Target-based azole resistance in Candida albicans involves overexpression of the ERG11 gene encoding lanosterol 14α-demethylase (LDM), and/or the presence of single or multiple mutations in this enzyme. The azole antifungals inhibit sterol 14α-demethylase (CYP51, SDM), thereby preventing biosynthesis of the essential and fungal specific sterol ergosterol, and resulting in the collateral synthesis of toxic sterols. We have used, as surrogates, structurally aligned mutations in recombinant hexahistidine-tagged full-length Saccharomyces cerevisiae LDM6×His (ScLDM6×His) to elucidate how differential susceptibility to azole drugs is conferred by LDM of the C. albicans Darlington strain. Phenotypes and high-resolution X-ray crystal structures were determined for the surrogate enzymes in complex with representative short-tailed (voriconazole) and long-tailed (itraconazole) triazoles.

Boat-shaped crystals of Ni-NTA affinity and size exclusion chromatography (SEC) purified ScLDM6×His Y140H in complex with VCZ formed after 15 days in 46% PEG, 0.5 M glycine pH 9.6. However, no active site water molecule was detected within 5 Å of VCZ in this 1.9 Å resolution structure, and the VCZ was displaced slightly towards H140 and helix I by <0.5 Å. Thus, there are no water-mediated hydrogen bond networks involving the tertiary alcohol of VCZ and Y140H and the heme ring D propionate, or between the 5-fluoropyrimidine ring and the main chain nitrogen of S382 and the main chain carbonyl of M509, as was found with the wild-type enzyme. The significantly different disposition of M509 between the wild-type and Y140H structures may be due to the absence of this water-mediated hydrogen bond network. There is also a significant impact on the disposition of Y126, which neighbors Y140/H, as the 5-fluoropyrimidine ring of VCZ was flipped 180 degrees between the wild-type and Y140H mutant structure. While the Y126 sidechain hydroxyl retained a hydrogen bond with the main chain amide of F384 in ScLDM6×His Y140H, a hydrogen bond with the heme ring D propionate was not formed. Due to the movement of VCZ towards helix I and the mutated histidine, the Y140H mutation ablates a key water-mediated hydrogen bond network involving the VCZ 5-fluoropyrimidine, the main chain amide of S382, and the main chain carbonyls of M509. While the ionic interactions of the heme with K151 and R385 were retained in ScLDM6×His Y140H, the loss of hydrogen bonds between Y140 and the heme ring C propionate, and between Y126 and the heme ring D propionate may be expected to affect the electronic status of the heme. This interpretation is consistent with the slight (1 nm) red shift from 417 nm to 418 nm in the main Soret peak of ScLDM6×His Y140H.

> MSATKSIVGEALEYVNIGLSHFLALPLAQRISLIIIIPFIYNIVWQLLYSLRKDRPPLVFYWIPWVGSAVVYGMKPYEFFEECQKKYGDIFSFVLLGRVMTVYLGPKGHEFVFNAKLADVSAEAAYAHLTTPVFGKGVIHDCPNSRLMEQKKFVKGALTKEAFKSYVPLIAEEVYKYFRDSKNFRLNERTTGTIDVMVTQPEMTIFTASRSLLGKEMRAKLDTDFAYLYSDLDKGFTPINFVFPNLPLEHYRKRDHAQKAISGTYMSLIKERRKNNDIQDRDLIDSLMKNSTYKDGVKMTDQEIANLLIGVLMGGQHTSAATSAWILLHLAERPDVQQELYEEQMRVLDGGKKELTYDLLQEMPLLNQTIKETLRMHHPLHSLFRKVMKDMHVPNTSYVIPAGYHVLVSPGYTHLRDEYFPNAHQFNIHRWNNDSASSYSVGEEVDYGFGAISKGVSSPYLPFGGGRHRCIGEHFAYCQLGVLMSIFIRTLKWHYPEGKTVPPPDFTSMVTLPTGPAKIIWEKRNPEQKIGGRHHHHHH> GGGMDYAKSDSSSLVTTMGEQFRSLRMLTRRSSPTDVLTGTSVTLPGITIGTDSSLRQSVLNIISYMYRFTKGSISYKIIPKIKGDLYITTSSADN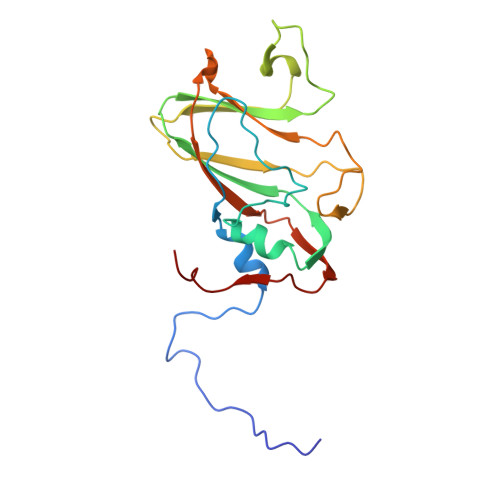IELNSNAYSFDVNRALHYQNTALNPVVQVSLPYYCPSENLVIDSTSFPNLSNLVLTNLERSSNTYTVLVSAGDDHTFSQLAGCPAFTIGPSRSAA Rotaviruses are the leading etiologic agent of viral gastroenteritis in infants and young children worldwide and are responsible for an estimated 140,000 deaths each year in developing countries. Diverse interactions between histo-blood group antigens (HBGAs) and rotavirus have been described and it is believed that HBGAs expressed on the surface of target cells serve as viral receptors. The distal VP8* portion (~27 kDa, N-terminal) of the rotavirus spike protein VP4 from P, P, P and P genotypes recognize the secretor HBGAs. To understand the molecular basis of LNB and H1 recognition and binding to P VP8* we determined the crystal structure of the clinical isolate P[8]c VP8* in its apo form and bound to LNB and H1 glycans.

Two different crystalline forms of P[8]c VP8* in its apo form were obtained. The first form, VP8*-Apo1, diffracts at 1.35 Å resolution and presents a single copy of P[8]c VP8* in the crystal asymmetric unit (ASU) while the second form, VP8*-Apo2, diffracts to 1.5 Å and presents two copies in the ASU. The three copies of P[8]c VP8* in these two crystalline forms present the galectin fold with two twisted β-sheets separated by a superficial cleft that conforms the glycan binding site in P and P genotypes. Superimposition of the individual VP8* protomers from these crystals showed that the three molecules of P[8]c VP8* are almost identical (RMSD 0.28 Å for the superposition of all the Cα). Furthermore, P[8]c VP8* are also structurally identical (RMSDs 0.37–0.57 Å) to the VP8* apo forms of the linage I P[8]Wa and P[8]Rotarix, supporting that the glycan binding site is preformed in the P[8]c VP8* protein.

> GSMLDGPYQPTTFTPPSDYWILINSNTNGVVYESTNNSDFWTAVIAVEPHVDPVDRQYNVFGENKQFNVRNDSDKWKFLEMFRGSSQNDFYNRRTLTSNTRLVGILKYGGRIWTFHGETPRATTDSSNTANLNGISITIHSEFYIIPRSQESKCNEYINNGL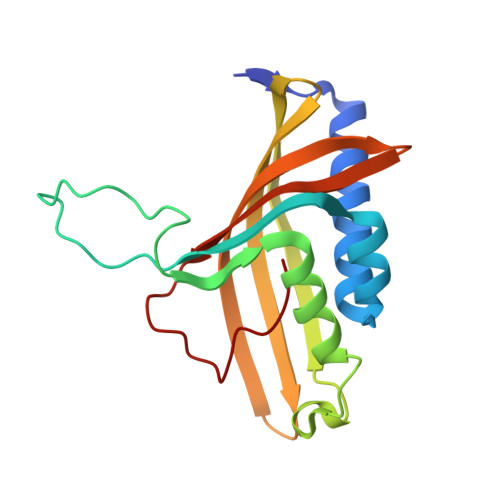> MSSEQIPVTPDVHYDIEAHYRAEVRMFQTGQYREWLQGMVAEDIHYWMPIYEQRLTRDRRPDPTPDDAAIYNDDFGELKQRVERLYSGQVWMEDPPSKIRYFVSNVEAFEAGNGELDVLSNILVYRNRRQTEVTVHTLGREDKLRRDGNGFKVFRRKLILDARVTQDKNLYFFC ACETYL PYRIDINE ADENINE DINUCLEOTIDE, REDUCED | C22 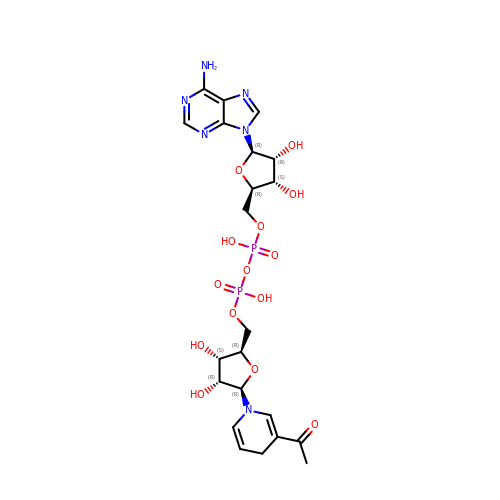H30 N6 O14 P2 | CIWXCGUGRDQCHH-RBEMOOQDSA-N> VFKKVLLTGTSEES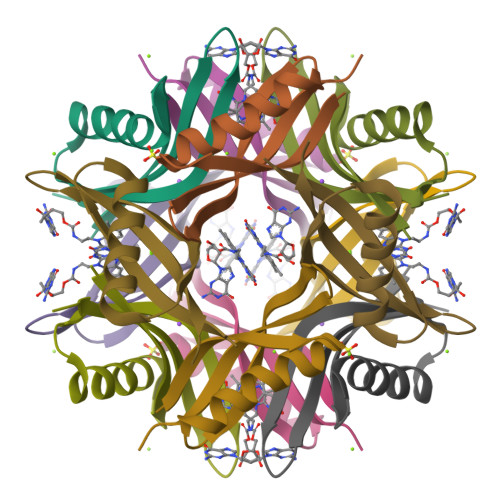FTAAADDAIDRAEDTLDNVVWAEVVDQGVAIGAVRTYQTEVQVAFELD> 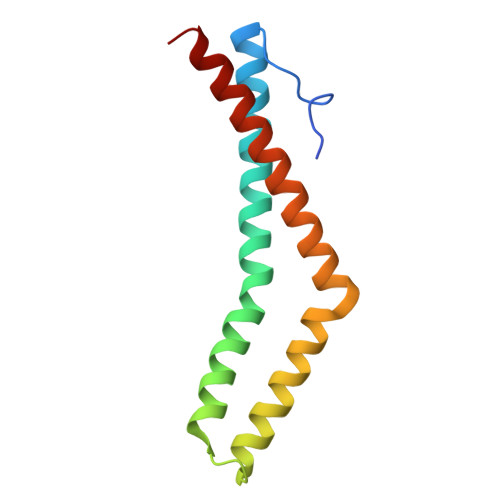GHMDEEWIREYPPITSDQQRQLYKRNFDTGLQEYKSLQSELDEINKELSRLDKELDDYREESEEYMAAADEYNRLKQVKGDADYKSKKNHCKQLKSKLSHIKKMVGDYDRQKT> MADDAIPHTDVLNSTAQGQLKSIIERVERLEVEKAEIMEQIKEVYAEAKGNGFDVKVLKKVVRIRKQDRAKRQEEDAILDLYLSAIGEILEHHHHH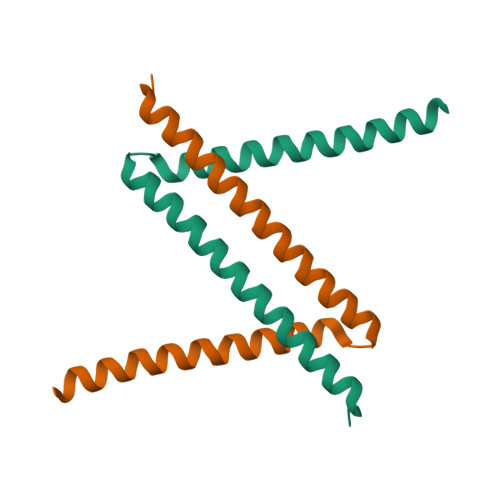H>APQQINDIVHRTITPLIEQQKIPGMAVAVIYQGKPYYFTWGYADIAKKQPVTQQTLFELGSVSKTFTGVLGGDAIARGEIKLSDPTTKYWPELTAKQWNGITLLHLATYTAGGLPLLVPDEVKSSSDLLRFYQNWQPAWAPGTQRLEANSSIGLFGALAVKPSGLSFEQAMQTRVFQPLKLNHTWINVPPAEEKNYAWGYREGKAVHVSPGALDAEAYGVKSTIEDMARWVQSNLKPLDINEKTLQQGIQLAQSRYWQTGDMYQGLGWEMLDWPVNPDSIINGS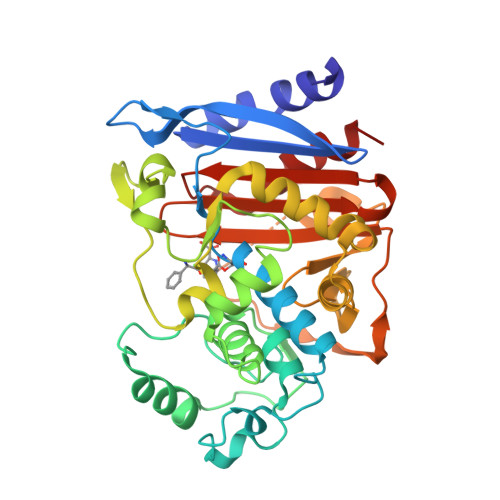DNKIALAARPVKAITPPTPAVRASWVHKTGATGGFGSYVAFIPEKELGIVMLANKNYPNPARVDAAWQILNALQ[2x]The second principal receptor for IgE, CD23, is a type II transmembrane glycoprotein with a C-type lectin-like domain (CTLD)4 (3, 4). In its membrane-bound form, CD23 consists of three CTLD “heads” connected to the membrane via a trimeric α-helical coiled-coil “stalk”. The interaction between CD23 and IgE is critical in the regulation of IgE synthesis, which can be up- or down-regulated depending on the oligomerization state of CD23 (2, 9, 10). We have determined the crystal structures of the human lectin-like head domain of CD23 in its Ca2+-free and Ca2+-bound forms, as well as the crystal structure of the Ca2+-bound head domain of CD23 in complex with a subfragment of IgE-Fc consisting of the dimer of Cϵ3 and Cϵ4 domains (Fcϵ3-4).

As predicted from the crystal structure, the introduction of the S252A mutation did not affect Ca2+ binding, but unexpectedly, the D258A mutant was unable to bind Ca2+ even though the aspartate forms part of the apparently nonfunctioning auxiliary Ca2+-binding site. D258A (auxiliary) and D270A (principal site) crystallized differently, and in all eight and seven molecules within the asymmetric unit, respectively, Pro-250 is trans. Mutation of Asp-258, which faces Pro-250 at the base of loop 4, to alanine results in a conformational change in loop 4 and a reorientation of Arg-253 compared with the Ca2+-free derCD23 structure; this was seen in all eight molecules within the asymmetric unit. The side chain of Arg-253 flips ∼180° and projects into the principal Ca2+-binding site cavity, occupying the Ca2+ ion position. The re-positioned Arg-253 side chain forms two salt bridges with the carboxylate group of Glu-249. Occupation of the Ca2+-binding site by Arg-253 explains why the D258A mutant fails to bind Ca2+. However, the crystal structure of this mutant, in contrast to the other three structures that all showed perturbations only at the site of mutation, revealed that the D258A mutation (at the base of loop 4) caused a major reorientation of Arg-253 such that its guanidinium group occupied the principal Ca2+-binding site.

>SGFVCNTCPEKWINFQRKCYYFGKGTKQWVHARYACDDMEGQLVSIHSPEEQDFLTKHASHTGSWIGLRNLDLKGEFIWVDGSHVDYSNWAPGEPTSRSQGEACVMMRGSGRWNDAFCDRKLGAWVCDRLATCTPPASEGSAE[8x]PROTOPORPHYRIN IX | C34 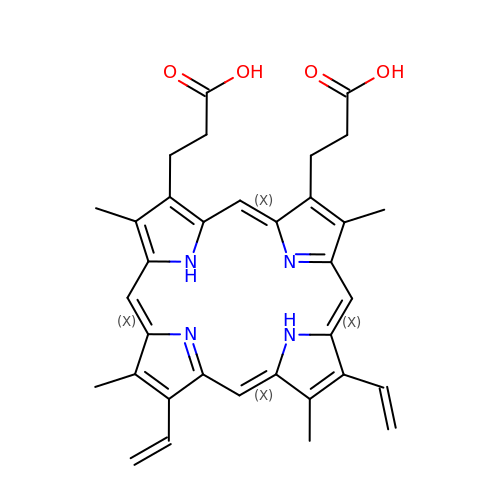H34 N4 O4 | FEDYMSUPMFCVOD-UJJXFSCMSA-N> MDLLAELQWRGLVNQTTDEDGLRKLLNEERVTLYCGFDPTADSLHIGHLAPILTMRRFQQAGH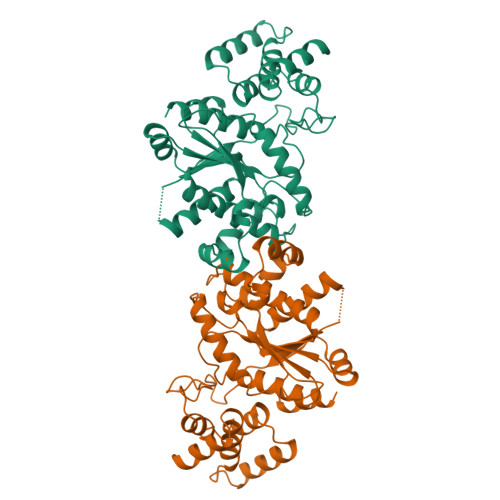RPIALVGGATGLIGDPSGKKSERTLNAKETVEAWSARIKEQLGRFLDFEADGNPAKIKNNYDWIGPLDVITFLRDVGKHFSVNYMMAKESVQSRIETGISFTEFSYMMLQAYDFLRLYETEGCRLQIGGSDQWGNITAGLELIRKTKGEARAFGLTIPLVTKADGTKFGKTESGTIWLDKEKTSPYEFYQFWINTDDRDVIRYLKYFTFLSKEEIEALEQELREAPEKRAAQKTLAEEVTKLVHGEEALRQAIRIS3-({3-[(2S)-2-amino-2-carboxyethyl]-5-bromo-2,6-dioxo-3,6-dihydropyrimidin-1(2H)-yl}methyl)thiophene-2-carboxylic 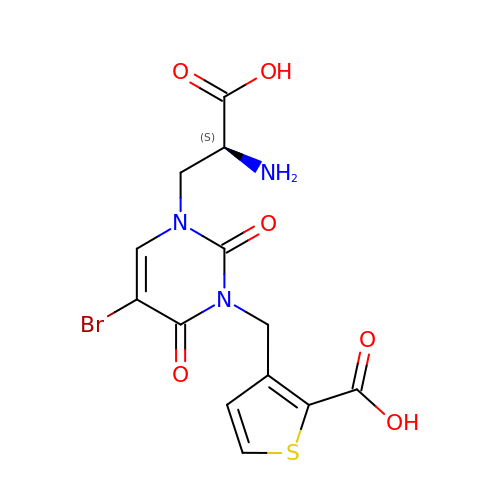acid | C13 H12 Br N3 O6 S | KKTBJRLDYITGOV-QMMMGPOBSA-N> GHMSETNTIFKLEGVSVLSPLRKKLDLVFYLSNVDGSPVITLLKGNDRELSIYQLNKNIKMASFLPVPEKPNLIYLFMTYTSCEDNKFSEPVVMTLNKENTLNQFKKLGLLDSNVTDFEKCVEYIRKQAILTGFKISNPFVNSTLVDTDAEKINSFHLQCHRGTKEGTLYFLPDHIIF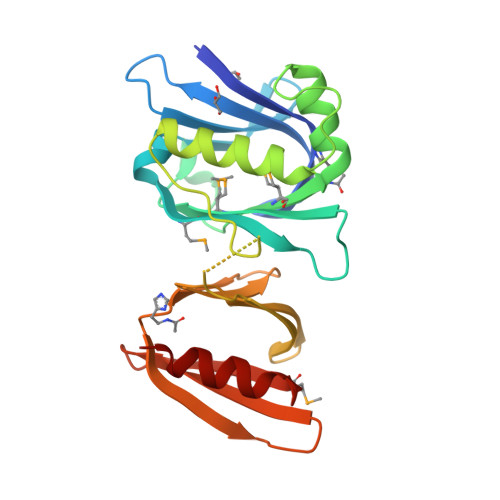GFKKPILLLDASDIESITYSSITRLTFNASLVTKDGEKYEFSMIDQTEYAKIDDYVKRK> GCCG

Ru–dipyridophenazine (dppz) complexes are of particular interest, because they are able to act as DNA probes or can induce guanine oxidation when exposed to light. The structures contain Λ‐[Ru(bpy)2(dppz)]2+ (1), Λ‐[Ru‐ (phen)2(dppz)]2+ (2) and Λ‐[Ru(phen)2(dppz‐11,12‐Me)]2+ (3) bound to a non‐self‐complementary DNA duplex of sequence d((5‐BrC)GGC) (strand 1) with d(GCCG) (strand 2). In all three structures, the complex intercalates into the 5′‐(5‐BrCG)‐3′ step with a canted binding mode.

At the binding site, the long axis of the dppz group is offset from the base hydrogen bonds by 44° on one side and 90° on the other and the complex is intercalated from the minor groove. The twist angle at the intercalation site is 28°, a reduction of 8° compared to standard B‐DNA. In all three structures, the complex is bound with one ancillary group (bpy/phen) packed against G4 on strand 2, resting against the backbone and hydrogen atom on the (G4)2 NH2 group. A consequence of binding is that between C3 and G4 on strand 2, the backbone elongates with a γ torsion angle of 153° instead of its standard angle of approximately 60°, creating an asymmetric cavity. The second ancillary group packs against (strand 1) G2 and (strand 2) C3. The dppz group sits directly above the C−G hydrogen bonds and is not directed towards either base. The structure of the binding site and DNA is virtually identical in structures 1–3 and, therefore, they will be discussed as a single entity from now on. However, the fact that they are so similar shows that there is little difference in binding between bpy and phen‐based Λ complexes and that methyl‐substitution at the 11th and 12th positions on the dppz does not change how the compounds bind, which is consistent with the crystal structure of Λ‐[Ru(TAP)2(dppz‐11,12‐Me)]2+ bound to d(TCGGCGCCGA)2. This observation shows that, as long as no major structural changes are made, Λ‐Ru‐dppz complexes can be treated as a single class of compound when it comes to their binding specificity. Luminescent life‐times, binding enthalpy and nearest neighbour cooperativity parameters are very similar for Λ‐[Ru(phen)2(dppz)]2+ and Λ‐[Ru(bpy)2(dppz)]2+ binding to [poly(dA‐dT)]2.>MTRILAPIPSPPKHPQYGHLHYLAGDAPVLNFFQLARQIPEGLFQLDIQGRTLIQAYDPNLVAELTDERRFQKRVHPAYTNIRNLGGDGLFTSDSFEPNWGKAHRILLPAFSQRAMKGYFGQMLEVAQALVGKWERTQGQDVRVADDMTRLTLDTISLSGFDYRFRSFDKDELHPFLQALARAMHHTMTMNSRPPVLTPEMEEADRAYWADIASMNELVDEVIRERRGHGGGGGDLLGLMLNATDPETGERLSDENIRYQVMTFLIAGHETTSGLLAFTLYLLLRHPHVLAQAYAEVDRLLPGDAVPTYDTVMRLDVIPRILDEALRFWSTIPNYAVTALQDEVIGGKYEIRKGQQVALLIPALHRHPA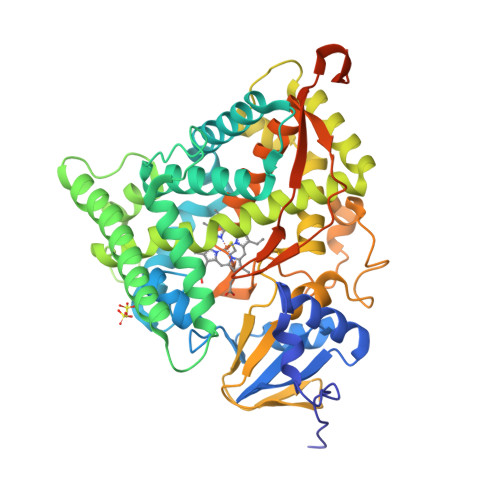AWTNPDEFDIDRWTSENRRTHHPAAYKPFGNGMRACIGRQFALTEAKLALLLILQKFALSDPYDYHLKVKQSLTIKPEDFALRVRERRPHERFSVPVPVVEEPQQDLSRVSVAGTGVALTVAYGLEHHHHHH[4x]> HDCV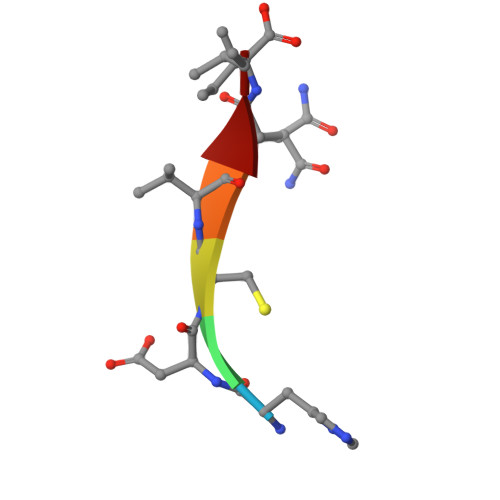NI> AAPGSVVELLGKSYPQDDHSNLTRKVLTRVGRNLHNQQHHPLWLIKERVKEHFYKQYVGRFGTPLFSVYDNLSPVVTTWQNFDSLLIPADHPSRKKGDNYYLNRTHMLRAHTSAHQWDLLHAGLDAFLVVGDVYRRDQIDSQHYPIFHQLEAVRLFSKHELFAGIKDGESLQLFEQSSRSAHKQETHTMEAVKLVEFDLKQMLTRLMAHLFGDELEIRWVDCYFPFTHPSFEMEINFHGEWLEVLGCGVMEQQLVNSAGAQDRIGWAFGLGLERLAMILYDIPDIRLFWCEDERFLKQFCVSNINQKVKFQPLSKYPAVINDISFWLPSENYAENDFYDLVRTIGGDLVEKVDLIDKFVHPKTHKTSHCYRITYRHMERTLSQREVRHIHQALQEAAVQLLGVEGRF

Mutations in the mitochondrial aminoacyl‐tRNA synthetases (mtaaRSs) can cause profound clinical presentations, and have manifested as diseases with very selective tissue specificity. Among the recently reported pathogenic variants are point mutations in FARS2 gene, encoding the human mitochondrial PheRS. Patient symptoms range from spastic paraplegia to fatal infantile Alpers encephalopathy. How clinical manifestations of these mutations relate to the changes in three‐dimensional structures and kinetic characteristics remains unclear, although impaired aminoacylation has been proposed as possible etiology of diseases.

Here, we report four crystal structures of HsmtPheRS mutants, and extensive MD simulations for wild‐type and nine mutants to reveal the structural changes on dynamic trajectories of HsmtPheRS. Using steady‐state kinetic measurements of phenylalanine activation and tRNAPhe aminoacylation, we gained insight into the structural and kinetic effects of mitochondrial disease‐related mutations in FARS2 gene.> VEDATRSDSTTQMSSTPEVVYSSAVDSKQNRTSDFDANWKFMLSDSVQAQDPAFDDSAWQQVDLPHDYSITQKYSQSNEAESAYLPGGTGWYRKSFTIDRDLAGKRIAINFDGVYMNATVWFNGVKLGTHPYGYSPFSFDLTGNAKFGGENTIVVKVENRLPSSRWYSGSGIYRDVTLTVTDGVHVGNNGVAIKTPSLATQNGGDVTMNLTTKVANDTEAAANITLKQTVFPKGGKTDAAIGTVTTASKSIAAGASADVTSTITAASPKLWSIKNPNLYTVRTEVLNGGKVLDTYDTEYGFRWTGFDATSGFSLNGEKVKLKGVSMHHDQGSLGAVANRRAIERQVEILQKMGVNSIRTTHNPAAKALIDVCNEKGVLVVEEVFDMWNRSKNGNTEDYGKWFGQAIAGDNAVLGGDKDETWAKFDLTSTINRDRNAPSVIMWSLGNEMMEGISGSVSGFPATSAKLVAWTKAADSTRPMTYGDNKIKANWNESNTMGDNLTANGGVVGTNYSDGANYDKIRTTHPSWAIYGSETASAINSRGIYNRTTGGAQSSDKQLTSYDNSAVGWGAVASSAWYDVVQRDFVAGTYVWTGFDYLGEPTPWNGTGSGAVGSWPSPKNSYFGIVDTAGFPKDTYYFYQSQWNDDVHTLHILPAWNENVVAKGSGNNVPVVVYTDAAKVKLYFTPKGSTEKRLIGEKSFTKKTTAAGYTYQVYEGSDKDSTAHKNMYLTWNVPWAEGTISAEAYDENNRLIPEGSTEGNASVTTTGKAAKLKADADRKTITADGKDLSYIEVDVTDANGHIVPDAANRVTFDVKGAGKLVGVDNGSSPDHDSYQADNRKAFSGKVLAIVQSTKEAGEITVTAKADGLQSSTVKIATTAVPGTSTE;> AVDSKQNRTSDFDANWKFMLSDSVQAQDPAFDDSAWQQVDLPHDYSITQKYSQSNEAESAYLPGGTGWYRKSFTIDRDLAGKRIAINFDGVYMNATV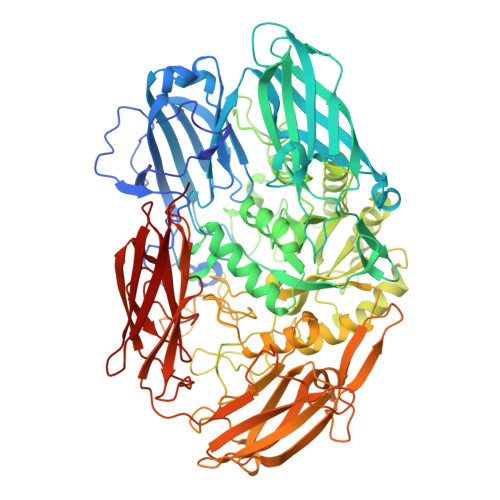WFNGVKLGTHPYGYSPFSFDLTGNAKFGGENTIVVKVENRLPSSRWYSGSGIYRDVTLTVTDGVHVGNNGVAIKTPSLATQNGGDVTMNLTTKVANDTEAAANITLKQTVFPKGGKTDAAIGTVTTASKSIAAGASADVTSTITAASPKLWSIKNPNLYTVRTEVLNGGKVLDTYDTEYGFRWTGFDATSGFSLNGEKVKLKGVSMHHDQGSLGAVANRRAIERQVEILQKMGVNSIRTTHNPAAKALIDVCNEKGVLVVEEVFDMWNRSKNGNTEDYGKWFGQAIAGDNAVLGGDKDETWAKFDLTSTINRDRNAPSVIMWSLGNEMMEGISGSVSGFPATSAKLVAWTKAADSTRPMTYGDNKIKANWNESNTMGDNLTANGGVVGTNYSDGANYDKIRTTHPSWAIYGSETASAINSRGIYNRTTGGAQSSDKQLTSYDNSAVGWGAVASSAWYDVVQRDFVAGTYVWTGFDYLGEPTPWNGTGSGAVGSWPSPKNSYFGIVDTAGFPKDTYYFYQSQWNDDVHTLHILPAWNENVVAKGSGNNVPVVVYTDAAKVKLYFTPKGSTEKRLIGEKSFTKKTTAAGYTYQVYEGSDKDSTAHKNMYLTWNVPWAEGTISAEAYDENNRLIPEGSTEGNASVTTTGKAAKLKADADRKTITADGKDLSYIEVDVTDANGHIVPDAANRVTFDVKGAGKLVGVDNGSSPDHDSYQADNRKAFSGKVLAIVQSTKEAGEITVTAKADGLQSSTVKIATTAVP~{N}-[4-(6,7-dimethoxyquinolin-4-yl)oxy-3-fluoranyl-phenyl]-4-ethoxy-1-(4-fluoranyl-2-methyl-phenyl)pyrazole-3-carboxamide 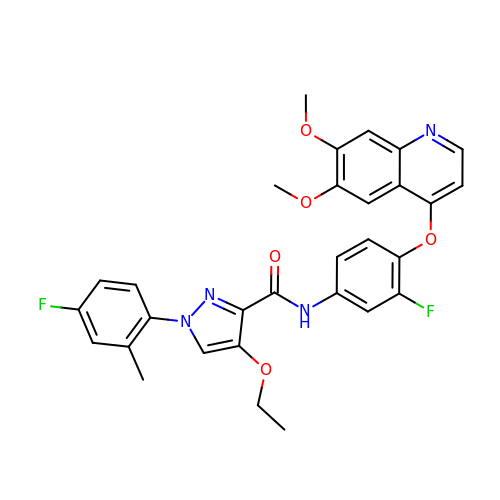| C30 H26 F2 N4 O5 | ISPBCAXOSOLFME-UHFFFAOYSA-N>MDYGMYFFEHVTPYETLVRRMERVIASGKTPFQDYFLFESKGFGKVLILDKDVQSTERDEYIYHETLVHPAMLTHPEPKRVLIVGGGEGATLREVLKHPTVEKAVMVDIDGELVEVAKRHMPEWHQGAFDDPRAVLVIDDARAYLER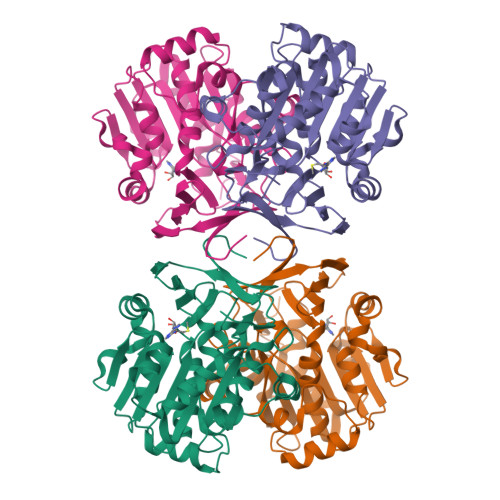TEERYDVVIIDLTDPVGEDNPARLLYTVEFYRLVKAHLNPGGVMGMQAGMILLTHHRVHPVVHRTVREAFRYVRSYKNHIPGFFLNFGFLLASDAFDPAAFSEGVIEARIRERNLALRHLTAPYLEAMFVLPKDLLEALEKETMVSTDQNPFYVTPEGEARQAPYKG[2x]N-ethyl-N'-(1-methylethyl)-6-(methylsulfanyl)-1,3,5-triazine-2,4-diamine | C9 H17 N5 S | 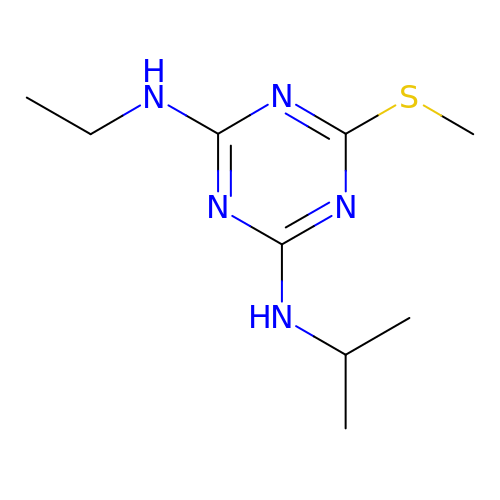RQVYBGPQFYCBGX-UHFFFAOYSA-N(2R)-2-cyclopropyl-5-methyl-2-[3-(5-prop-1-yn-1-ylpyridin-3-yl)phenyl]-2H-imidazol-4-amine 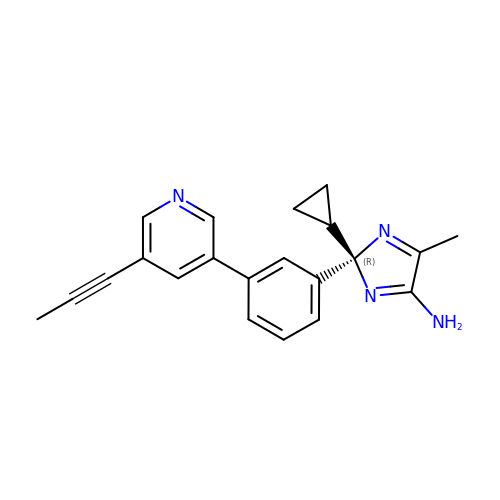| C21 H20 N4 | TWHSRVVFCICXII-OAQYLSRUSA-N> MHHHHHHLVPRGSMLDFEKPLFEIRNKIESLKESQDKNDVDLQEEIDMLEASLERETKKIYTNLKPWDRVQIARLQERPTTLDYIPYIFDSFMELHGDRNFRDDPAMIGGIGFLNGRAVTVIGQQRGKDTKDNIYRNFGMAHPEGYRKALRLMKQAEKFNRPIFTFIDTKGAYPGKAAEERGQSESIATNLIEMASLKVPVIAIVIGEGGSGGALGIGIANKVLMLENSTYSVISPEGAAALLWKDSNLAKIAAETMKITAHDIKQLGIIDDVISEPLGGAHKDIEQQALAIKSAFVAQLDSLESLSRDEIANDRFEKFRNIGSYIE;> MFKDFFNRTKKKKYLTVQDSKNNDVPAGIMTKCPKCKKIMYTKELAENLNVCFNCDHHIALTAYKRIEA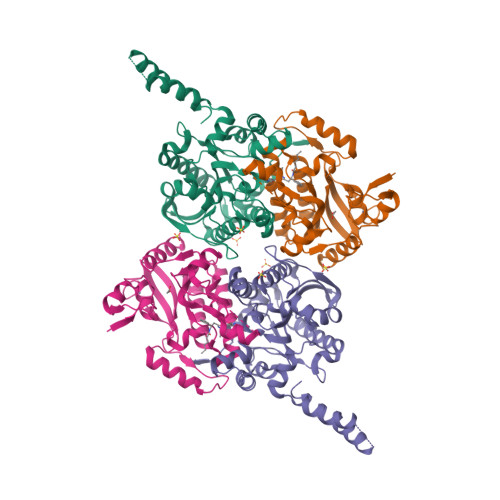ISDEGSFTEFDKGMTSANPLDFPSYLEKIEKDQQKTGLKEAVVTGTAQLDGMKFGVAVMDSRFRMGSMGSVIGEKICRIIDYCTENRLPFILFSASGGARMQEGIISLMQMGKTSVSLKRHSDAGLLYISYLTHPTTGGVSASFASVGDINLSEPKALIGFAGRRVIEQTINEKLPDDFQTAEFLLEHGQLDKVVHRNDMRQTLSEILKIHQEVTK>[2x]GPLGSPEFQKTKPFSVPNLPLNTLSNSRVPSLINAMMISRDHGQMVQFQNGRVTLDGQLQGTTPTSLSQLCKIRGKVFHASGGNGLNLTELDGSAYHAFESPAPIGFPDIGDCDWHMSATATNNFTGSSNEYQILIKQESAFAPHLGHVQADNLSAGANTDLIVSLSWISPVSDQHRHDVDPWVIPRYGSSLTEAAQLAPPIYPPGFGEAIVFFMSDFPVVSGVNGMRIPCTLPQEYVAHFVNEQAPTRGEAALLHYVDPDTHRNLGEFKMYPEGFMTCVPNSSGSGPQTLPINGVFTFVSWVSRFYQLKPVGTAGPARRLGIRRS

NoV VP1 can be divided into two major domains: the N-terminal shell (S) domain and the C-terminal protruding (P) domain. The P domains form the outermost, dimeric protrusions of NoV virions, which plays critical roles in receptor recognition and host immune responses. HuNoVs recognize human histo-blood group antigens (HBGAs) as host receptors or attachment factors that play an important role in huNoV host susceptibility. In this study, we provided both phenotypic and structural evidence to show that huNoV DSV and VA115 recognize a group of glycans with terminal galactoses as ligands.

The crystal structure of the native DSV P protein was solved at 2.10 Å resolution, containing a homodimer in the crystallographic asymmetric unit. All DSV P protein residues (228–531) were built in electronic density map. The two P proteins exhibited the typical huNoV P dimer arch-like structure with the P1 subdomains situated at the bottom and the P2 subdomain situated at the top. The major structural differences compared with other known P proteins are at the surface exposed loops, including the previously identified A-, B-, P-, T-, and U-loops in the P2 subdomain and the S-loop in the P1 subdomain. These variable loops confer DSV and VA115 unique surface topology from other huNoVs. We noted that the P-loop and T-loop on the surface of DSV/VA115 P protein exhibit a higher extension and the distance between the two loops becomes closer. Therefore, the glycan binding pocket becomes narrower but deeper, which hinders the binding to HBGAs. Through structural superimposition of the DSV P domain and HBGA oligosaccharides with other known structures, we found that the α-acetylgalactosamine (GalNAc), the A epitope, and α-Gal of the B epitope are too close to the amino acids on the T-loop, resulting in an obvious chemical steric hindrance. Similar clash also occurs between the α-1,2 fucose of the H-type trisaccharide and the S346′ amino acid residue on the P-loop. Likewise, the representative α-1,3/4 fucose of Lewis antigen forms a clash with Y439′ on the S-loop.> LSPDAYRFLTELDRQLRLLQAQIQRLLEAQSL

Here, we probe the mechanism of oligomerization of a peptide representing the CCD of the STIL protein, a tetrameric multi-domain protein that is over-expressed in several cancers and associated with metastatic spread. STIL tetramerization is mediated both by an intrinsically disordered domain (STIL400–700) and a structured CCD (STIL CCD718–749). The STIL protein plays a highly important role in mitosis by regulating centrosomal duplication. The CCD of STIL is necessary for its self-association.

Two-point mutations (A722L and Q729L) and a double mutant of these (A722L + Q729L) were designed. Both of these sites are predicted as d positions in the coiled-coil heptad repeats, and as leucine (Leu, L) predominates at these positions in natural coiled coils we changed the Ala (A) and Gln (Q) to that residue. AUC-SV experiments at 10 µM for these mutants all returned solution-phase molecular weights consistent with tetramers, and at 100 µM the data and fits were even more robust. A722L had a cooperative unfolding transition with a Tm of over 70 °C, and Q729L and the A722L + Q729L double mutant did not undergo thermal denaturation. CCD mutants bearing these two substitutions as well as the double mutant A722L + Q729L formed very stable anti-parallel tetramers, which could not be dissociated under any experimental conditions. We also solved a structure of Q729L to 1.66 Å resolution. This revealed an anti-parallel tetramer, which we describe as a dimer of dimers. The interaction between the monomers in the dimer is tighter than the interactions between the two dimers. Likewise, the packing in central portion of the tetrameric bundle is tighter than the ends. Aligning the Q729L dimer to the L736E dimer resulted in mean RMSD of 1.6 ± 0.5 Å (over an average of 58 Cα atoms), indicating that the dimeric and tetrameric states are more structurally related than the biological assembly of the previously determined structure of the STIL CCD (cyan).>[2x]MDSSRTIGLYFDSALPSSNLLAFPIVLQDIGDGKKQIAPQYRIQRLDSWTDSKEDSVFITTYGFIFQVGNEEVTVGMISDNPKHELLSAAMLCLGSVPNVGDLVELARACLTMVVTCKKSATDTERMVFSVVQAPQVLQSCRVVANKYSSVNAVKHVKAPEK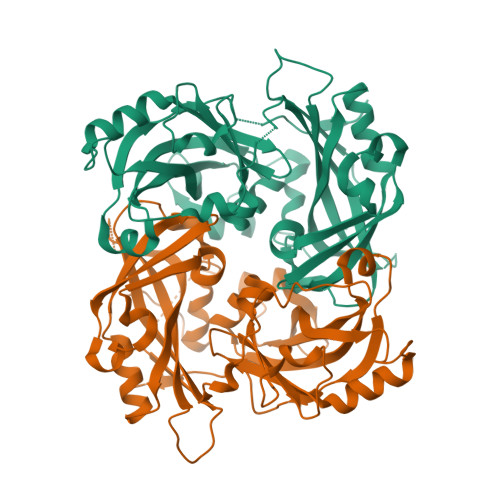IPGSGTLEYKVNFVSLTVVPRKDVYKIPTAALKVSGSSLYNLALNVTIDVEVDPKSPLVKSLSKSDSGYYANLFLHIGLMSTVDKKGKKVTFDKLERKIRRLDLSVGLSDVLGPSVLVKARGARTRLLAPFFSSSGTACYPISNASPQVAKILWSQTARLRSVKVIIQAGTQRAVAVTADHEVTSTKIEKRHTIAKYNPFKK>[2x]NLYFQGMVTKIIWVSNNGKPNLKIEFVSEEEKSNFFKEVKKKASELGLNFPLVQGSGNSLLIEASNYPINPCGCYISPGGKLAINFGKVELSHFILPKVGVKTEHAEIFK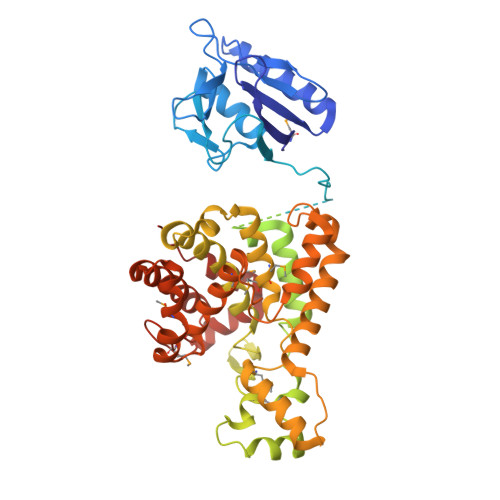DHNTIFFHKHKLPGVNSELTFIPTGTPVIVPVTKPATTSPAFFNPSKSGDSSISISAIGNVDSPMIRITFQNQTEREFFLNKITDKAKSLGVNISTHPFEIKEPNMVLIKPSKYPDNKLGCYISKNKEIAINFGRTDFRDFVLSNLGVGSHLGTCPTKNETGNDTFYFHQENLSLNGPALSVNTKITKEIEKNDYLLSANGSKAIDFVWSNFLKHPYNPKLKQPDANVKAAWEKHADWEHWSNMGQDWSLNTPSGLVPRPNHGIAHTLRVAQLVPVIAEFLKAYSGDPKFQKLTQKEIQKAQYMMLFSVIGRENDMSWTDANHYQQAFKEAYNGQYSKHIYATFKENAQKGFLNHVVTNKSSLIPSLFSDESELQYWAEALDTGKPGISSASGILMALAHDLDLMRCYDKGKFNSLKMKDLVARLGGNEDAAKKLADYAHDLIVATGDRCMGYGVTQDYNYSLFGKCSLDPNECLKQLQSIPKPETTLANQYGI>SPPQKVCLICGDEASGCHYGVLTCEGCKAFFKRAVEGQHNYLCAGRNDCIIDKIRRKNCPACRLRKCLQAGMTLGARKSKK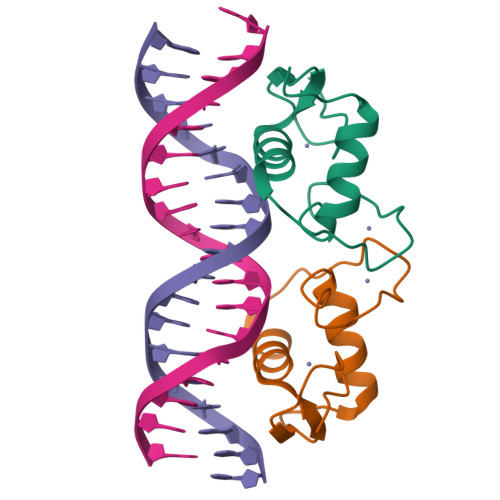L[4x]(2~{S})-1-[(3~{S})-3-[[(3~{S})-3,4-bis(oxidanyl)-4-oxidanylidene-butyl]amino]-4-oxidanyl-4-oxidanylidene-butyl]azetidine-2-carboxylic 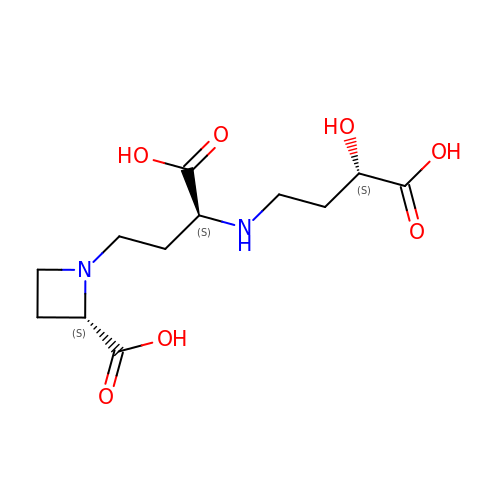acid | C12 H20 N2 O7 | CUZKLRTTYZOCSD-CIUDSAMLSA-N>MELWLVRHGETLWNREGRLLGWTDLPLTAEGEAQARRLKGALPSLPAFSSDLLRARRTAELAGFSPRLYPELREIHFGALEGALWETLDPRYKEALLRFQ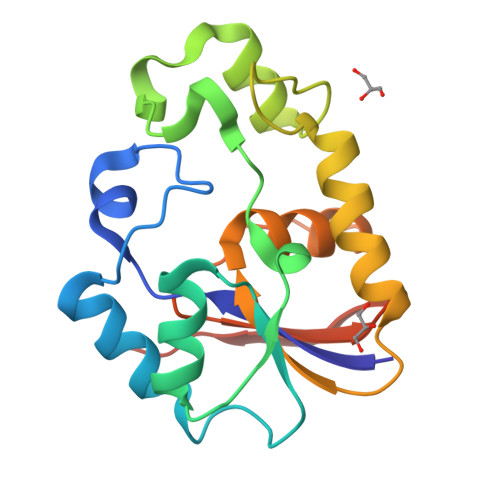GFHPPGGESLSAFQERVFRFLEGMKAPAVLFTHGGVVRAVLRALGEDGLVPPGSAVAVDWPRRVLVRLALDGEEATG[2x]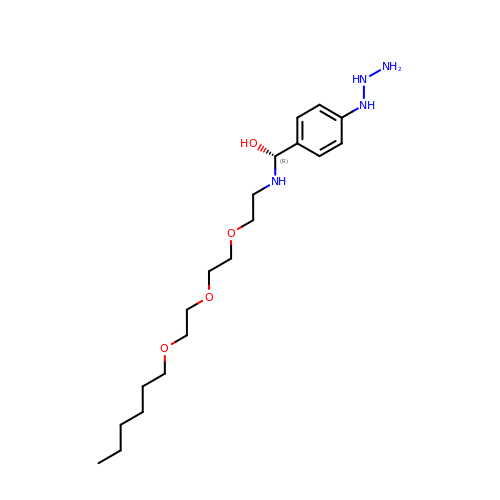(R)-[4-(2-azanylhydrazinyl)phenyl]-[2-[2-(2-hexoxyethoxy)ethoxy]ethylamino]methanol | C19 H36 N4 O4 | LFWZOPMQWFRAFE-LJQANCHMSA-N> GAMSFSSNSSSDTNSILYAGPTFTHSP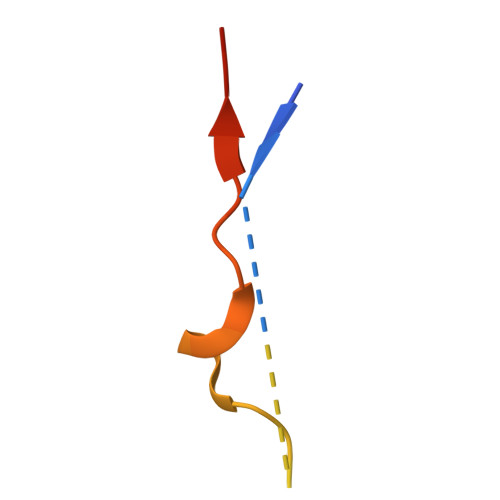AASNLPIPTFLHSP> MKHHHHHHMKQNSPLDEENLTQENQDRGTHVDRGLASANVDFAFSLYKQLVLKAPDKNVIFSPLSISTALAFLSLGAHNTTLTEILKGLKFNLTETSEAEIHQSFQHLLRT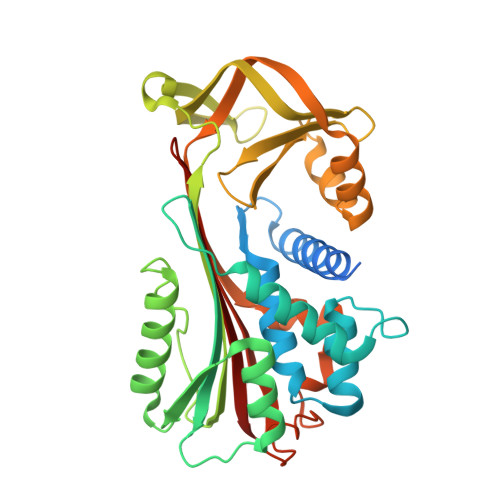LNQSSDELQLSMGNAMFVKEQLSLLDRFTEDAKRLYGSEAFATDFQDSAAAKKLINDYVKNGTRGKITDLIKDLDSQTMMVLVNYIFFKAKWEMPFDPQDTHQSRFYLSKKKWVMVPMMSLHHLTIPYFRDEELSCTVVQLNYTGNASALFILPDQDKMEEVEAMLLPETLNRWGDSLEFREIGELYLPKFSISRDYNLNDILLQLGIEEAFTSKADLSGITGARNLAVSQVVHKAVLDVFEEGTEASAATAVKITLL>[2x]MPIHDKSPRPQEFAAVDLGSNSFHMVIARVVDGAMQIIGRLKQRVHLADGLGPDNMLSEEAMTRGLNCLSLFAERLQGFSPASVCIVGTHTLRQALNATDFLKRAEKVIPYPIEIISGNEEARLIFMGVEHTQPEKGRKLVIDIGGGSTELVIGENFEPILVESRRMGCVSFAQLYFPGGVINKENFQRARMAAAQKLETLTWQFRIQGWNVAMGASGTIKAAHEVLMEMGEKDGIITPERLEKLVKEVLRHRNFASLSLPGLSEERKTVFVPGLAILCGVFDALAIRELRLSDGALREGVLYEMEGRFRHQDVRSRTASSLANQYHIDSEQARRVLDTTMQMYEQWREQQPKLAHPQLEALLRWAAMLHEVGLNINHSGLHRHSAYILQNSDLPGFNQEQQLMMATLVRYHRKAIKLDDLPRFTLFKKKQFLPLIQLLRLGVLLNNQRQATTTPPTLTLITDDSHWTLRFPHDWFSQNALVLL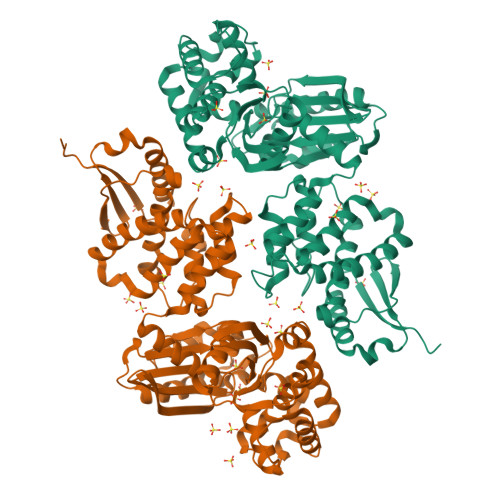DLEKEQEYWEGVAGWRLKIEEESTPEIAA Interleukin 4 (IL-4) is a pleiotropic cytokine that plays a major regulatory role in the immune system. Signal transduction of IL-4 is mediated by a sequential binding process, initiated first by binding of IL-4 to its high-affinity single membrane spanning receptor chain IL-4Rα. This intermediate ligand receptor complex then recruits one of two possible low-affinity receptor subunits, the common gamma chain (γc) or the IL-13Rα1 chain, into the functional hetero-trimeric complex to initiate signalling. The overall structure of IL-4 comprises the known four-helical bundle in up-up-down-down topology, which like the crystal packing is unaffected by these mutations.

We tested the interaction model proposed above by mutating Arg85 of IL-4 and the super-agonistic variants to alanine and measuring the residual binding affinity to IL-4Rα. If Arg85 is really involved in generating the additional stability/interaction, then, owing to cooperativity, mutation of this residue would have a greater effect in the super-agonistic variants (decrease in binding affinity) compared to wild-type IL-4. In contrast, the affinity of the IL-4 variant T13D-R85A is decreased 6.5-fold and its dissociation rate reflects IL-4 wild-type-like binding kinetics. An even bigger effect is observed for the variant F82D-R85A. Here the equilibrium binding constant is increased almost 36-fold, mainly because of the increased dissociation rate (koff (F82D-R85A)/koff (F82D) ~ 9). To exclude the possibility that structural changes in addition to the removal of the Arg85 side chain play a role in the changes in binding stability, we determined the structures of the IL-4 variants R85A, T13D-R85A and F82D-R85A. No changes in the local structure around residues Thr/Asp13, Phe/Asp82 or Arg85 could be observed (data not shown).

> HKCDITLQEIIKTLNSLTEQKTLCTELTVTDIFAASKNTTEKETFCRAATVLRQFYSHHEKDTRCLGATAQQFHRHKQLIRDLKALDRNLWGLAGLNSCPVKEANQSTLENFLERLKTIMREKYSKCSS> GASLKDFELSKMLEKVAKESSVGTPRAINEDILDQGYTVEGNQLINHLSVRASHAERMRSNPDSVRSQLGDSV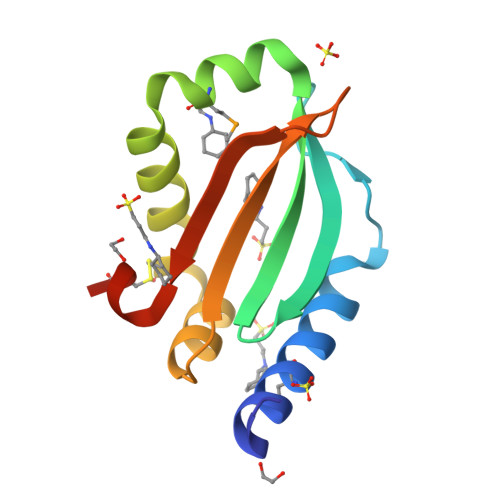CSNTGYRQLLARGAILTYSFTEYKTNQPVATERFDAGSCRIQGKK>[41x]TLEELRAEARILEAKAEILKAKAEVLKAKAEILKAQ

Here we report seven high-resolution cryo-EM structures of filamentous peptide nanotubes based on a cross-α supramolecular architecture that provide insight into the designability of helical peptide filaments. A structural interaction is identified based on an appropriately placed pair of arginine residues (RxxxR) within the corresponding peptide sequences. This local interaction motif, designated as an arginine clasp, is robust within the context of these cross-α assemblies and can guide the coalescence of helical protofilaments into structurally defined cross-α nanotubes. In contrast to most structurally characterized filaments based on synthetic α-helical coiled-coils, the chain axes of the helical protomers are oriented in a plane nearly perpendicular to the long axis of the assembly.

In a control experiment, a second computational optimization was performed in which positions 6, 7, 10, and 36 were constrained to those in the original peptide sequence. The arginine residues at positions 6 and 10 defined the RxxxR motif, while residues at positions 7 and 36 (Ala and Gln, respectively) appeared to be important for organizing this motif. A comparison between the two sequences, 36-31-3_LL and 36-31-3_RR, could provide additional insight into importance of structural preservation of the arginine clasp interaction. The computationally designed peptides, 36-31-3_LL and 36-31-3_RR, displayed an α-helical conformation and formed high aspect-ratio filaments of similar width to those of 36-31-3. In contrast, 36-31-3_RR filaments persisted over weeks in solution. The differences in stability between the two computationally designed filaments suggested that the cohesive interactions were much weaker in the absence of the arginine clasp interaction. In order to confirm that the arginine clasp was conserved, filaments of 36-31-3_RR were analyzed by cryo-EM. A 4.5-Å resolution reconstruction of the 36-31-3_RR filaments displayed a nearly identical structure to that of the original 36-31-3 filaments, with very slight differences in the rise (2.49 versus 2.51 Å/subunit) and the rotation (124.5 versus 124.0 degrees/subunit) for the respective 1-start helices of the 3D models. Accordingly, repeating the statistical analysis of this assembly’s RxxxR motif produced very similar results as for the original 36-31-3 filament, indicating the native rarity of the geometry.>MATKSVLQPPAAGSASIVGGAGGTQLLPKNISQEWWKKATEQSIIPTLSKSTPVIIGDGNVVPVLTKRPSASIIGELQNKVDSELEVGAKNFKTIKAEVGLEFSLETILTNPAGILDIIGEEMSGALARQVDAAVIHNRQSSNGAQLTSGTVSITAGAPTVELPLTAGVDIDPFLWEGYNTVTEAAGNNFSGFAFDPRLTYVLATARDSDGRRLNPDINMGQTVTSYSGQPAINSRTVGGDVDAGTDTGIRAIGGDWDALRFGYAHQIGLRKIEYGDPFGNGDLQRRNAVAYLMEVIFGWVVLDPNAF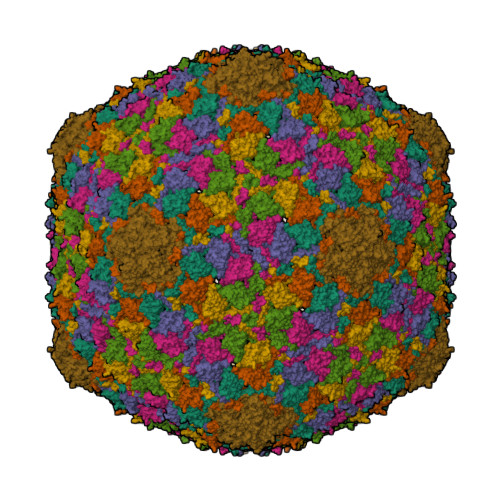VVYKLAAEDEEPETP[7x]> GTESKKMSSELFTLTYGALVTQLCKDYENDEDVNKQLDRMGYNIGVRLIEDFLARSNVGRCHDFRETADVIAKVAFKMYLGITPSITNWSPAGDEFSLILEN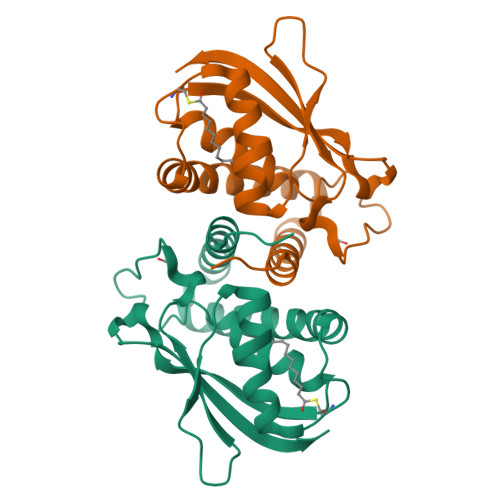NPLVDFVELPDNHSALIYSNLLCGVLRGALEMVQMAVEAKFVQDTLKGDGVTEIRMRFIRRIE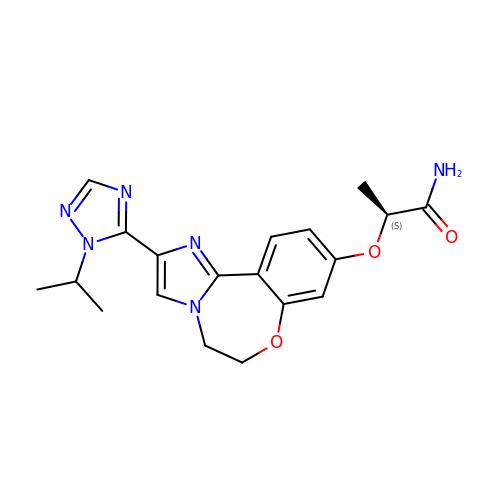(2S)-2-({2-[1-(propan-2-yl)-1H-1,2,4-triazol-5-yl]-5,6-dihydroimidazo[1,2-d][1,4]benzoxazepin-9-yl}oxy)propanamide | C19 H22 N6 O3 | SIKYDKLGPWRPMZ-LBPRGKRZSA-N>MAAAAQNLQKKVKNAKGIEVIYQSSYKGKIRPGQIKMTVSGNQVALESVSPKGEKETATEGIREDKQPVIKNYIDYAGREAYKWAELPDGKIISAATPFEFGKGFTPAGEGKHLGLNCKIARTSINSNTIEVWYTHDIPFRGTPQANVGVPDGLVLKVVRNGDMIQEASAITPLKKAQALLPDSWGEKMDAADYQYTINQSGVITIPVFDQQTICFNNAKLPDTLEDGITYSAGGGTLILKKVKLPESAKNRSIFVEVAQYSDGDAYDRTGSVFVIPTDKKQSFLDAIRNLKSVPSFQAKDGNYPALISTDDYEAPVELMRFFTGFGVRKFNHNKVKGQHWVDSVIYKSEVTPLASQLQGEVWIGAYIGNWDAKGHRLSLKLKYYPDDERRVNKAMPLFNTVNYLEQAGQAYPVFFLNDSLRVRFTLKEPAKNARLFYLTTGHGGWGNGDEFNQKPNTVYLDGKKVISFIPWR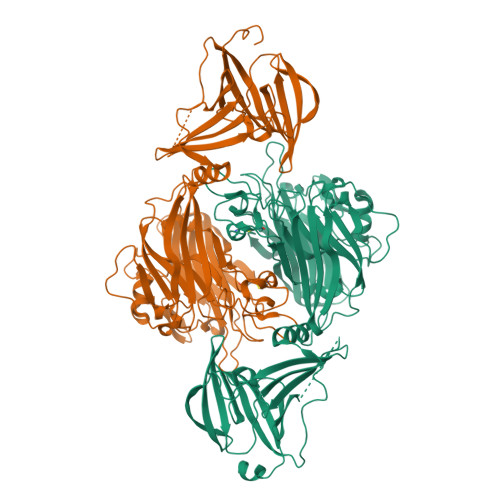DDCGTYRNSNPCSGNFSNGLSSSDLSRSNWCPGTVTTPEYIYLGDLEAGEHTLSVRIPQGAPEGGSNSYWCISGTLLYLEHHHHHH[2x]> FWST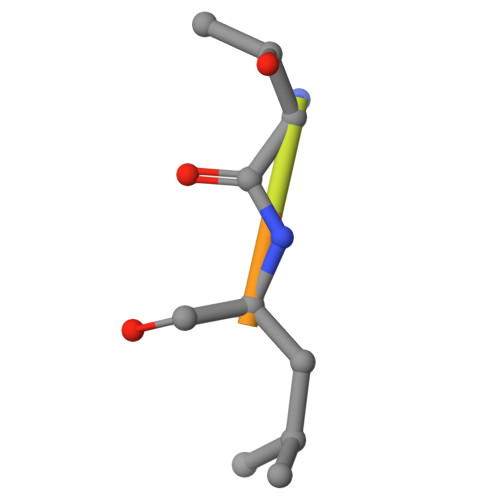LSPI> MELKHSISDYTEAEFLQLVTTICNADTSSEEELVKLVTHFEEMTEHPSGSDLIYYPKEGDDDSPSGIVNTVKQWRAANGKSGFKQG;> MESKRNKPGKATGKGKPVGDKWLDDAGKDSGAPIPDRIADKLRDKEFKSFDDFRKAVWEEVSKDPELSKNLNPSAKSSVSKGYSPFTPKNQQVGGRKVYELHHDKPISQGGEVYDMDNIRV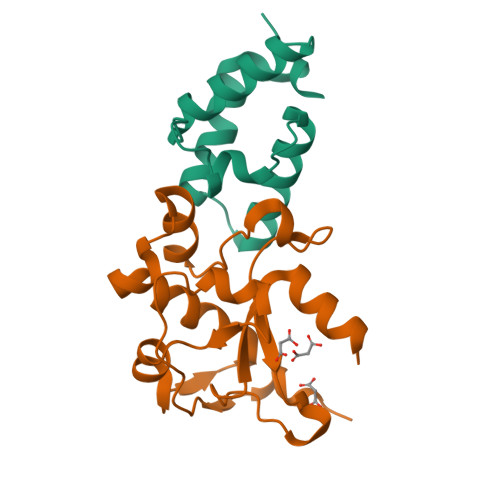TTPKRHIDIHRGK4-ethoxy-4-oxobutanoic acid | C6 H10 O4 | 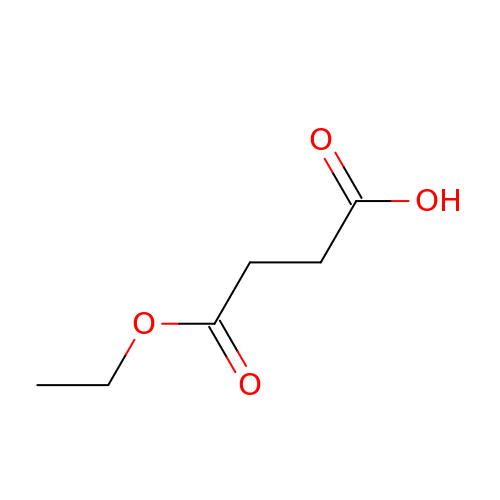LOLKAJARZKDJTD-UHFFFAOYSA-N>[3x]LKCNQLIPPFWKTCPKGKNLCYKMTMRAAPMVPVKRGCIDVCPKSSLLIKY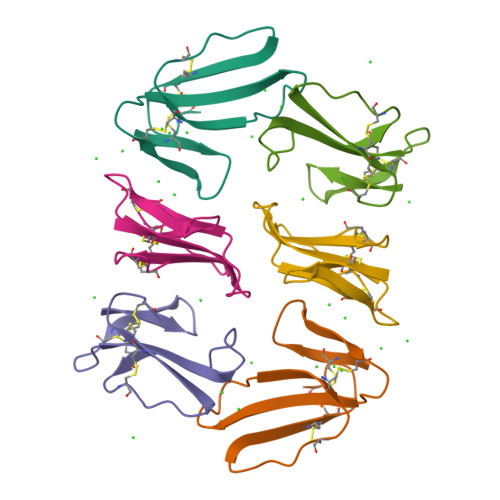MCCNTDKCN> NKKTAQLLHADTPRLVTWDAGLCTSFKIVPIVPAQVPQDVLAYTFFTSSYAIQSPFPEAAVSRIVVHTRWASNVDFDRDSSVIMAPPTENNIHLFKQLLNTETLSVRGANPLMFRANVLHMLLEFVLDNLYLNRHTGFSQDHTPFTEGANLRSLPGPDAEKWYSIMYPTRMGTPNVSKICNFVASCVRNRVGRFDRAQMMNGAMSEWVDVFETSDALTVSIRGRWMARLARMNINPTEIEWALTECAQGYVTVTSPYAPSVNRLMPYRISNAERQISQIIRIMNIGNNATVIQPVLQDISVLLQRISPLQIDPTIISNTMSTVSESTTQTLSPASSILGKLRPSNSDFSSFRVALAGWLYNGVVTTVIDDSSYPKDGGSVTSLENLWDFFILALALPLTTDPCAPVKAFMTLANMMVGFETIPMDNQIYTQSRRASAFSTPHTWPRCFMNIQLISPIDAPILRQWAEIIHRYWPNPSQIRYGAPNVFGSANLFTPPEVLLLPIDHQPANVTTPTLDFTNELTNWRARVCELMKNLVDNQRYQPGWTQSLVSSMRGTLDKLKLIKSMTPMYLQQLAPVELAVIAPMLPFPPFQVPYVRLDRDRVPTMVGVTRQSRDTITQPALSLSTTNTTVGVPLALDARAITVALLSGKYPPDLVTNVWYADAIYPMYADTEVFSNLQRDMITCEAVQTLVTLVAQISETQYPVDRYLDWIPSLRASAATAATFAEWVNTSMKTAFDLSDMLLEPLLSGDPRMTQLAIQYQQYNGRTFNVIPEMPGSVIADCVQLTAEVFNHEYNLFGIARGDIIIGRVQSTHLWSPLAPPPDLVFDRDTPGVHIFGRDCRISFGMNGAAPMIRDETGMMVPFEGNWIFPLALWQMNTRYFNQQFDAWIKTGELRIRIEMGAYPYMLHYYDPRQYANAWNLTSAWLEEITPTSIPSVPFMVPISSDHDISSAPAVQYIISTEYNDRSLFCTNSSSPQTIAGPDKHIPVERYNILTNPDAPPTQIQLPEVVDLYNVVTRYAYETPPITAVVMGVP;> AGLCTSFKIVPIVPAQVPQDVLAYTFFTSSYAIQSPFPEAAVSRIVVHTRWASNVDFDRDSSVIMAPPTENNIHLFKQLLNTETLSVRGANPLMFRANVLHMLLEFVLDNLYLNRHTGFSQDHTPFTEGANLRSLPGPDAEKWYSIMYPTRMGTPNVSKICNFVASCVRNRVGRFDRAQMMNGAMSEWVDVFETSDALTVSIRGRWMARLARMNINPTEIEWALTECAQGYVTVTSPYAPSVNRLMPYRISNAERQISQIIRIMNIGNNATVIQPVLQDISVLLQRISPLQIDPTIISNTMSTLSPASSILGKLRPSNSDFSSFRVALAGWLYNGVVTTVIDDSSYPKDGGSVTSLENLWDFFILALALPLTTDPCAPVKAFMTLANMMVGFETIPMDNQIYTQSRRASAFSTPHTWPRCFMNIQLISPIDAPILRQWAEIIHRYWPNPSQIRYGAPNVFGSANLFTPPEVLLLPIDHQPANVTTPTLDFTNELTNWRARVCELMKNLVDNQRYQPGWTQSLVSSMRGTLDKLKLIKSMTPMYLQQLAPVELAVIAPMLPFPPFQVPYVRLDRDRVPTMVGVTRQSRDTITQPALSLSTTNTTVGVPLALDARAITVALLSGKYPPDLVTNVWYADAIYPMYADTEVFSNLQRDMITCEAVQTLVTLVAQISETQYPVDRYLDWIPSLRASAATAATFAEWVNTSMKTAFDLSDMLLEPLLSGDPRMTQLAIQYQQYNGRTFNVIPEMPGSVIADCVQLTAEVFNHEYNLFGIARGDIIIGRVQSTHLWSPLAPPPDLVFDRDTPGVHIFGRDCRISFGMNGAAPMIRDETGMMVPFEGNWIFPLALWQMNTRYFNQQFDAWIKTGELRIRIEMGAYPYMLHYYDPRQYANAWNLTSAWLEEITPTSIPSVPFMVPISSDHDISSAPAVQYIISTEYNDRSLFCTNSSSPQTIAGPDKHIPVERYNILTNPDAPPTQIQLPEVVDLYNVVTRYAYETPPITAVVMGVP;>[2x]ARAAFLFKTVGFGGLQNVPINDELSSHLLRAGNSPWQLTQFLDWISLGRGLATSALVPTAGSRYYQMSCLLSGTLQIPFRPNHRWGDIRFLRLVWSAPTLDGLVVAPPQVLAQPALQAQADRVYDCDDYPFLARDPRFKHRVYQQLSAVTLLNLTGFGPISYVRVDEDMWSGDVNQLLMNYFGHTFAEIAYTLCQASANRPWEHDGTYARMTQIILSLFWLSYVGVIHQQNTYRTFYFQCNRRGDAAEVWILSCSLNHSAQIRPGNRSLFVMPTSPDWNMDVNLILSSTLTGCLCSGSQLPLIDNNSVPAVSRNIHGWTGRAGNQLHGFQVRRMVTEFCDRLRRDGVMTQAQQNQIEALADQTQQFKRDKLEAWAREDDQYNQANPNSTMFRTKPFTNAQWGRGNTGATSAAIAALI;>[3x]TINVTGDGNVFKPSAETSSTAVPSLSLSPGMLNPGGVPWIAIGDETSVTSPGALRRMTSKDIDEPLVVVTEHAIANFTKAEMALEFNREFLDKLRVLSVSPKYSDLLTYVDCYVGVSARQALNNFQKQVPVITPTRQTMYVDSIQAALKALEKWEIDLRVAQTLLPTNVPIGEVSCPMQSVVKLLDDQLPDDSLIRRYPKEAAVALAKRNGGIQWMDVSEGTVMNEAVNAVAASALAPSASAPPLEEKSKLTEQAMDLVTAAEPEIIASLVPVPAPVFAIPPKPADYNVRTLKIDEATWLRMIPKTMGTLFQIQVTDNTGTNWHFNLRGGTRVVNLDQIAPMRFVLDLGGKSYKETSWDPNGKKVGFIVFQSKIPFELWTAASQIGQATVVNYVQLYAEDSSFTAQSIIATTSLAYNYEPEQLNKTDPEMNYYLLATFIDSAAITPTNMTQPDVWDALLTMSPLSAGEVTVKGAVVSEVVPAELIGSYTPESLNASLPNDAARCMIDRASKIAEAIKIDDDAGPDEYSPNSVPIQGQLAISQLETGYGVRIFNPKGILSKIASRAMQAFIGDPSTIITQAAPVLSDKNNWIALAQGVKTSLRTKSLSAGVKTAVSKLSSSESIQNWTQGFLDKVSTHFPAP;> ANVWGVRLADSLSSPTIETRTRQYTLHDLCSDLDANPGREPWKPLRNQRTNNIVAVQLFRPLQGLVLDTQLYGFPGAFDDWERFMREKLRVLKYEVLRIYPISNYSNEHVNVFVANALVGAFLSNQAFYDLLPLLIINDTMIGDLLGTGASLSQFFQSHGDVLEVAAGRKYLQMENYSNDDDDPPLFAKDLSDYAKAFYSDTYEVLDRFFWTHDSSAGVLVHYDKPTNGHHYLLGTLTQMVSAPPYIINATDAMLLESCLEQFSANVRARPAQPVTRLDQCYHLRWGAQYVGEDSLTYRLGVLSLLATNGYQLARPIPRQLTNRWLSSFVSQIMSDGVNETPLWPQERYVQIAYDSPSVVDGATQYGYVRKNQLRLGMRISALQSLSDTPSPVQWLPQYTIDQAAMDEGDLMVSRLTQLPLRPDYGNIWVGDALSYYVDYNRSHRVVLSSELPQLPDTYFDGDEQYGRSLFSLARKIGDRSLVKDTAVLKHAYQAIDPNTGKEYLRSRQSVAYFGASAGHSGADQPLVIEPWIQGKISGVPPPSSVRQFGYDVAR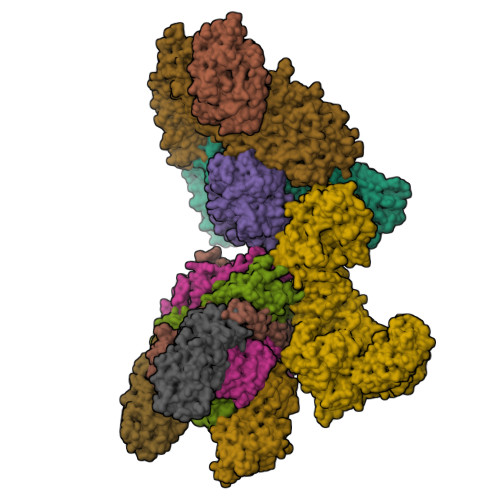GAIVDLARPFPSGDYQFVYSDVDQVVDGHDDLSISSGLVESLLSSCMHATAPGGSFVVKINFPTRPVWHYIEQKILPNITSYMLIKPFVTNNVELFFVAFGVHQHSSLTWTSGVYFFLVDHFYRYETLSTISRQLPSFGYVDDGSSVTGIETISIENPGFSNMTQAARIGISGLCANVGNARKSIAIYESHGARVLTITSRRSPASARRKSRLRYLPLIDPRSLEVQARTILPADPVLFENVSGASPHVCLTMMYNFEVSSAVYDGDVVLDLGTGPEAKILELIPATSPVTCVDIRPTAQPSGCWNVRTTFLELDYLSDGWITGVRGDIVTCMLSLGAAAAGKSMTFDAAFQQLIKVLSKSTANVVLVQVNCPTDVVRSIKGYLEIDSTNKRYRFPKFGRDEPYSDMDALEKICRTAWPNCSITWVPLSYDLRWTRLALLESTTLSSASIRIAELMYKYMPIMRIDIHGLPMEKRGNFIVGQNCSLVIPGFNAQDVFNCYFNSALAFSTEDVNAAMIPQVSAQFDATKGEWTLDMVFSDAGIYTMQALVGSNANPVSLGSFVVDSPDVDITDAWPAQLDFTIAGTDVDITVNPYYRLMTFVRIDGQWQIANPDKFQFFSTLVMNVKLDIADKYLLYYIRDVQSRDVGFYIQHPLQLLNTITLPTNEDLFLSAPDMREWAVKESGNTICILNSQGFVLPQDWDVLTDTISWSPSIPTYIVPPGDYTLTPL;>MEVCLPNGHQIVDLINNAFEGRVSIYSAQEGWDKTISAQPDMMVCGGAVVCMHCLGVVGSLQRKLKHLPHHRCNQQIRHQDYVDVQFADRVTAHWKRGMLSFVCQMHAMMNDVSPEDLDRVRTEGGSLVELNWLQVDPNSMFRSIHSSWTDPLQVVDDLDTKLDQYWTALNLMIDSSDLVPNFMMRDPSHAFNGVRLEGDARQTQFSRTFDSRSSLEWGVMVYDYSELEHDPSKGRAYRKELVTPARDFGHFGLSHYSRATTPILGKMPAVFSGMLTGNCKMYPFIKGTAKLKTVRKLVDSVNHAWGVEKIRYALGPGGMTGWYNRTMQQAPIVLTPAALTMFSDTTKFGDLDYPVMIGDPMILG[3x]> 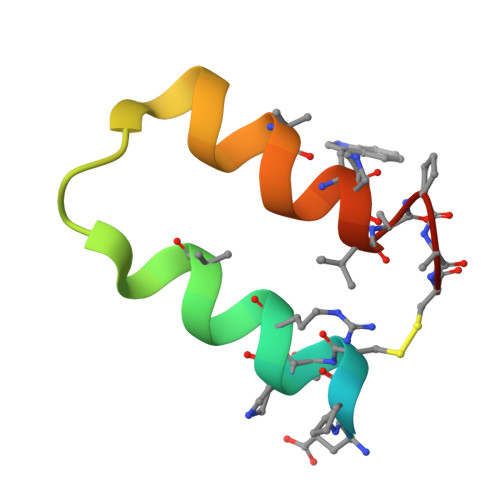VDNKXNKEXCNXRAIEAALDPNLNDQQFHAKIWXIIXDCX> ELEIEWHKFETSEEIISTYLIDDVLYTGVNGAVYTFSNNELNKTGLTNNNNYITTSIKVEDTLVCGTNNGNPKCWKIDGSEDPKYRGRGYAPYQNSKVTIISHNECVLSDINISKEGIKRWRRFDGPCGYDLYTADNVIPKDGVRGAFVDKDGTYDKVYILFTDTIDTKRIVKIPYIAQMCL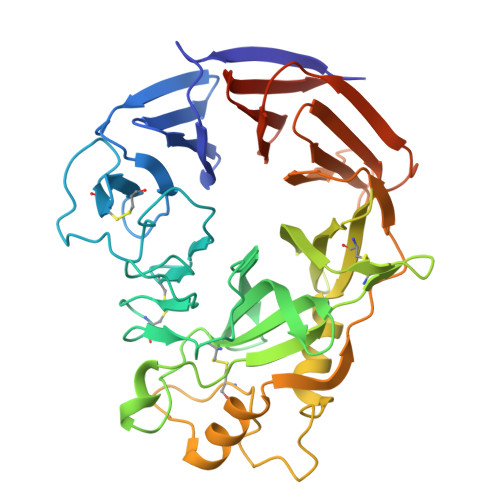NDEGGPSSLSSHRWSTFLKVELECDIDGRSYRQIIHSKAIKTDNDTILYVFFDSPYSKSALCTYSMNAIKHSFSTSKLGGYTKQLPSPAPGICLPAGKVVPHTTFDIIEQYNELDDIIKPLSQPIFEGPSGVKWFDIKEKENEHREYRIYFIKENTIYSFDTKSKQTRSAQVDARLFSVMVTSKPLFIADIGIGVGIPRMKKILKMGTHHHHHHHH>RVDDPAGKAAQYHKEYALFRSANMPSPDKLATGVGFHSFRIPAVVRTNTGRILAFAEGRRHNNRDYGDINLVYKRTKSPTNNGENPTDWESLREVVGTGPHTWGNPTPVVDGNTIYLFLSMNDGAYSQNGGNTLPDGTKTKKIDSTWVGRRHLY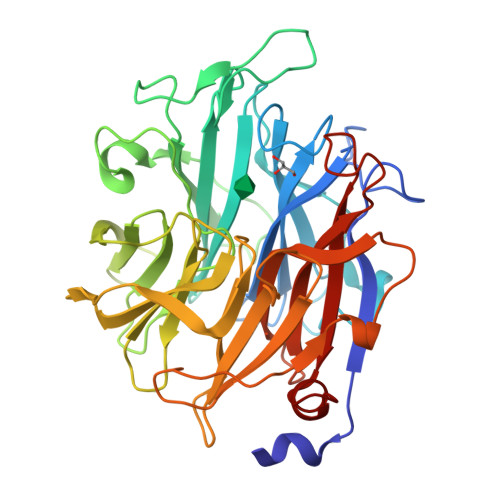LTTSTDDGDTWTKPVDMTKTLTPDGQAWDAVGPGNGIKLSTGELVIPAQGRNIIGRGPSGNRTWSMQILKGAGSEGTICQTPDGKLMRNDRPGPMGHRSVARGTLAGLGPFATDNGLPDPACQGSILSYNSDEPARTIFMNSASTDRRTAMRVRISYDKDAAKFNFGRELKDAPLGNVGNEGGYSSMTKTSDYKIGALVESDWYEDKGGEKSHRCIIWRRFNLSWIINGPNN[2x]> VRVSIERLWSQYFEARAKLGSLEPDEREAAETLEKRVRGLKDRLVVNYSPLVKYAAGRVTARSTGAVDQEEILSWGILGLLDAVETFDAGKGAKFETYAISKIKWAILDELRRLDXXXXXXXXXXXEAAEIEELRRNLVEAIKNLAERERLVTTFYFYEGLTLREIGKALGLTEGRISQILRQSLGKLRDSLSEPRTS;>MGEETYEGTSGREGGRHEEEVETRAARESAEEVWGGTEDLTSLSVEELKGLLARFDEEEKRISYRRRVIQGRIDVIRAEIVRRGGAVLSPEELARVLMGDVGDESEGGASGDRRGDGA[2x]

The RsiG–WhiG cognate pair is the only known example of a σ–anti-σ complex that is targeted by c-di-GMP. Here we show that the same σ–(c-di-GMP)–anti-σ switch has been co-opted during evolution to regulate distinct biological functions in unicellular and filamentous bacteria, controlling type IV pilus production in the genus Rubrobacter and the differentiation of reproductive hyphae into spores in Streptomyces. Moreover, we show that the anti-σ likely originated as a homodimer and evolved to become a monomer through an intragenic duplication event. Structural analyses revealed that these single-motif RsiGs form an antiparallel coiled-coil through homodimerization, enabling them to bind c-di-GMP in the same manner as the monomeric twin-motif RsiGs.

Thus, to elucidate how a single-motif homodimeric RsiG interacts with c-di-GMP and its partner WhiG protein, we solved the crystal structure of the R. radiotolerans (Rr) RsiG bound to c-di-GMP and Rr WhiG to 2.93-Å resolution. The R. radiotolerans complex contains one WhiGRr molecule, a c-di-GMP dimer, and a RsiGRr homodimer. In the complex, the RsiGRr forms the same antiparallel coiled-coil homodimer as observed in the apo RsiGRr structures. Because no c-di-GMP was added prior to crystallization, the c-di-GMP molecules seen in the Rr (RsiG)2–(c-di-GMP)2–WhiG structure copurified with the complex from the E. coli expression system. The bound c-di-GMP dimer is coordinated by two RsiGRr E(X)3S(X)2R(X)3Q(X)3D repeat motifs, with the same arrangement of contacts as observed in the Sv RsiG–(c-di-GMP)2–WhiG structure, but again, in this case each motif is provided by each subunit of the RsiGRr homodimer. However, in contrast to the S. venezuelae structure, which shows no contacts from the WhiG σ4 domain to c-di-GMP, the WhiGRr σ4 domain makes extensive contacts to the c-di-GMP. As noted, in the R. radiotolerans structure the WhiGRr σ4 domain is shifted relative to the S. venezuelae structure such that it directly abuts the c-di-GMP molecules, positioning residues Thr237, R239, and K243 from the α11 helix of σ4 to directly contact the bound c-di-GMP dimer. In addition, the Rr RsiG homodimeric coiled-coil, though similar to the coiled-coil in the RsiGSv monomer, lacks the long interfacing loop seen in RsiGSv. Instead, RsiGRr employs N-terminal and C-terminal extensions from its coiled-coil to bind WhiGRr. The Rr (RsiG)2–(c-di-GMP)2–WhiG structure revealed how sequence-identical regions of the two RsiG subunits can flexibly adopt different conformations, allowing them to interact with distinct WhiGRr σ2 and σ4 domains.> MKQELEVLTANIQDLKE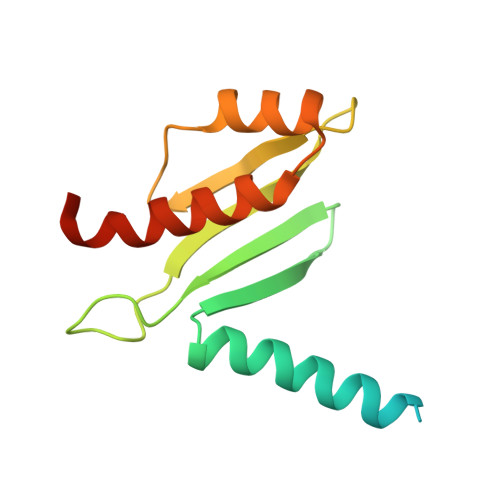EYSRKKETISTANKANAERLKRLQKSADLYKDRLGLEIRKIYGEKLQFIFTNIDPKNPESPFMFSLHLNEARDYEVSDSAPHLEGLAEFQENVRKTNNFSAFLANVRKAFTATVYNHHHHHH Sirtuins are NAD+-dependent protein lysine deacylases implicated in metabolic regulation and aging-related dysfunctions. Sirt1 features the conserved sirtuin catalytic core of ~270 residues, which comprises a Rossman-fold domain and a smaller Zn2+-binding module. A cleft between these subdomains accommodates NAD+ and recognizes the acylated substrate polypeptide with low sequence selectivity, and binding of these substrates is accompanied by Sirt1 closure movements. Tat binds to the sirtuin catalytic core and inhibits Sirt1, Sirt2, and Sirt3 with comparable potencies.

We, thus, used Sirt3 as a model system for structural analysis of the sirtuin/Tat interaction and resolved the crystal structure of a Sirt3/Tat-37–59 complex at 1.95 Å resolution. The structure was refined to Rcryst/Rfree values of 22.7/27.6% and revealed clear electron density for part of the peptide ligand. Consistent with the kinetic data, the inhibitory Tat fragment occupies the sirtuin substrate peptide channel but does not overlap with the NAD+ site. Best defined in the inhibitory peptide is a small fragment, residues 48–52, which belongs to the Tat basic domain, while residues 44–47 and 53–57 are primarily defined via their peptide backbone. The complete basic motif assumes an extended conformation, terminated by Pro58. This conformation resembles the generic sirtuin–substrate interaction, which comprises a four-residue substrate stretch in β-strand conformation inserted between the β8-α9 loop and the β6-α8 loop of the sirtuin. The sirtuin-bound Tat conformation also resembles the conformation of this Tat region in NMR structures of the apo forms of wt-Tat and Tat-Cys−, indicating that the appropriate conformation for sirtuin binding is intrinsically preferred and this Tat region, thus, “primed” for sirtuin binding. The Tat peptide assumes a binding mode deviating from substrates (see below), however, N- and C-terminally from this basic core, supported by charge complementarity. While the N-terminus binds at a positively charged sirtuin surface patch, the C-terminal basic motif with its positive charges occupies a strongly negatively charged sirtuin pocket. Although it is not acetylated, inhibitory Tat Lys50 is positioned in the sirtuin substrate lysine pocket.

>[2x]SDKGKLSLQDVAELIRARACQRVVVMVGAGISTPSGIPDFRSPGSGLYSNLQQYDLPYPEAIFELPFFFHNPKPFFTLAKELYPGNYKPNVTHYFLRLLHDKGLLLRLYTQNIDGLERVSGIPASKLVEAHGTFASATCTVCQRPFPGEDIRADVMADRVPRCPVCTGVVKPDIVFFGEPLPQRFLLHVVDFPMADLLLILGTSLEVEPFASLTEAVRSSVPRLLINRDLVGPLAWHPRSRDVAQLGDVVHGVESLVELLGWTEEMRDLVQRETGKLDGPDK;>AFITKGLGISYGRKKRRQRRRPS[2x]From yeast to mammals, the SET1 and MLL-like (mixed-lineage leukemia) multi-subunit protein complexes, known as SET1 or MLL COMPASS, are responsible for H3K4 methylation. Dpy30 is an important subunit of MLL/SET1 complexes, where it plays an essential role in both catalyzing H3K4 trimethylation and maintaining the state of trimethylated H3K4. Dpy30 directly interacts with Ash2L in human (Bre2 in yeast) COMPASS through its Dpy30-binding motif (DBM). Although the structures of the human Dpy30 C-terminal domain (Dpy30C) and SPRY domain of Ash2L containing the DBM motif were solved, the binding mode and stoichiometry of Dpy30 and Ash2L within COMPASS remain uncertain, partly because the complex structure is lacking.

We also solved the Dpy30 full-length (Dpy30FL) structure at a resolution of 2.13 Å. It contains two Dyp30 molecules in an asymmetric unit. Although we used the Dpy30FL sample for crystallization, only the C-terminal 55 residues (amino acids 45–99) were well defined in the structure. The C-terminal domains of two Dpy30 monomers form a semi-circle hydrophobic groove, accommodating a helix with poorer electron density. We can only model a fragment of poly-alanine here without visible side chains based on the electron density map. We deduced that this fragment could be the Dpy30 N-terminal domain because no other peptide was mixed with the protein during purification and crystallization. One N-terminal helix was bound in the hydrophobic groove of the neighboring Dpy30C dimer. However, it is noteworthy that the binding site is exactly the same as that observed for the Dpy30C dimer (CD) interacting with the Bre2DBM peptide. The molecular packing pattern of the Dpy30FL crystal indicates that Dpy30 oligomerizes with weak stability. In the Dpy30FL structure, a Dpy30C dimer binds with one target peptide; thus, the packing pattern presents a hexamer model of Dpy30 interacting with target helices at a ratio of 4:2.

>[2x]MEPEQMLEGQTQVAENPHSEYGLTDNVERIVENEKINAEKSSKQKVDLQSLPTRAYLDQTVVPILLQGLAVLAKERPPNPIEFLASYLLKNKAQFEDRNLERPHRD>SNAMRVLTGLQPSGDLHIGNYFGAIKQMVDAQEKSQMFMFIANYHAMTSSQDGEKLKQNSLKAAAAFLSLGIDPQKSVFWLQSDVKEVMELYWILSQFTPMGLLERAHSYKDKVAKGLSASHGLFSYPVLMAADILLFDTRIVPVGKDQIQHVEIARDIALKVNNEWGEIFTLPEARVNEEVAVVVGTDGAKMSKSYQNTIDIFSSEKTLKKQISSIVTDSTALEDPKDHENCNIFKIAKLFLDESGQKELQIRYEKGGEGYGHFKIYLNELVNAYFKEAREKYNELLEKPSHLKEILDFGAT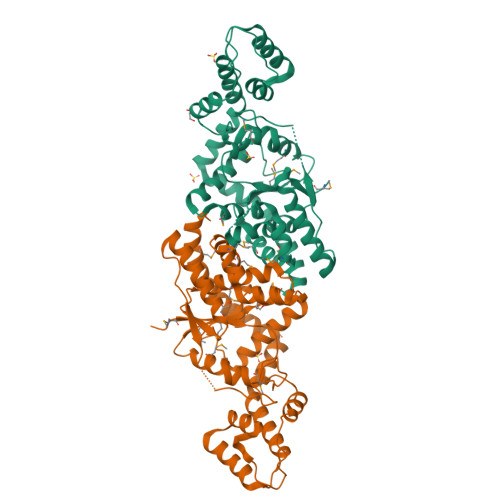KARKIAQEKMQKIYEKIGL[2x]>[8x]MSLKIRDAYTIVTCPGRNFVTLKIVTESGTHGIGDATLNGREMAVAAYLDEHVVPALIGRDAGRIEDTWQYLYRGAYWRRGPVTMTAIAAVDMALWDIKAKAAGMP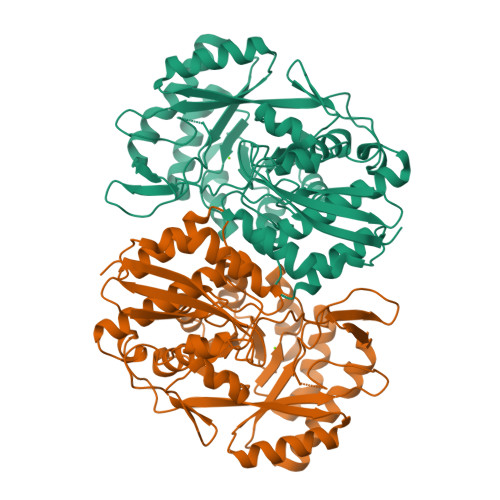LYQLLGGKSRERVMTYAHCTGQTIEDCLGEVARHVELGYRAVRVQSGVPGIETTYGVAKTPGERYEPADSSLPAEHVWSTEKYLNHAPKLFAAVRERFGDDLHVLHDVHHRLTPIEAARLGKAVEPYHLFWLEDCVPAENQESLRLIREHTTTPLAIGEVFNSIHDCRELIQNQWIDYIRMPLTHGGGITAMRRVADLASLYHVRTGFHGPTDLSPVCLGAAIHFDTWVPNFGIQEHMPHTDETDAVFPHDYRFEDGHFLAGESPGHGVDIDEELAAKYPYERASLPVNRLEDGTLWHW5-chloro-7-hydroxy-6-(phenylmethyl)pyrazolo[1,5-a]pyrimidine-3-carbonitrile 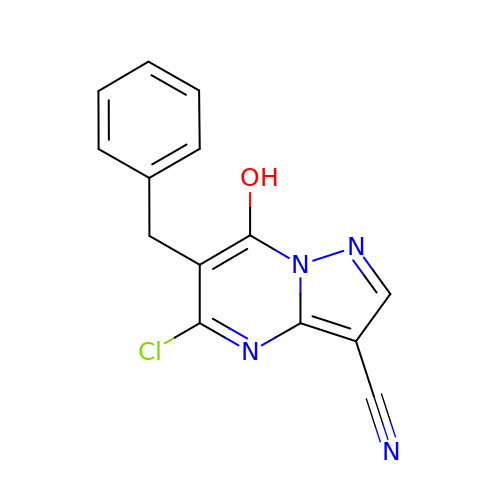| C14 H9 Cl N4 O | HOHNWEMSRSQMGQ-UHFFFAOYSA-N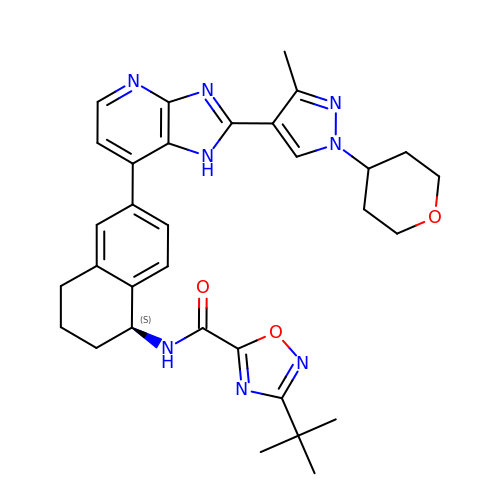3-tert-butyl-N-[(1S)-6-{2-[3-methyl-1-(oxan-4-yl)-1H-pyrazol-4-yl]-1H-imidazo[4,5-b]pyridin-7-yl}-1,2,3,4-tetrahydronaphthalen-1-yl]-1,2,4-oxadiazole-5-carboxamide | C32 H36 N8 O3 | ZJVGDVFZOUURTK-VWLOTQADSA-N>MKHLHRFFSSDASGGIILIIAAILAMIMANSGATSGWYHDFLETPVQLRVGSLEINKNMLLWINDALMAVFFLLVGLEVKRELMQGSLASLRQAAFPVIAAIGGMIVPTLLYLAFNYADPITREGWAIPAATDIAFALGVLALLGSRVPLALKIFLMALAIIDDLGAIIIIALFYTNDLSMASLGVAAVAIAVLAVLNLCGARRTGVYILVGVVLWTAVLKSGVHATLAGVIVGFFIPLKEKHGRSPAKRLEHVLHPWVAYLILPLFAFANAGVSLGGVTLDGLTSILPLGIIAGMLIGKPLGISLFCWLALRLKLAHLPEGTTYQQIMVVGILCGIGFTMSIFIASLAFGSVDPELINWAKLGILVGSISSAVIGYSWLRVRLRPSVGSENLYFQ[2x]

Na+/H+ exchangers facilitate the exchange of monovalent cations (Na+/Li+/K+) and protons (H+) across membranes to regulate intracellular pH, sodium levels and cell volume. Na+/H+ exchangers that perform this task are physiological homodimers, and whilst the ion transporting domain is highly conserved, their dimerization differs. The transporter is made up of two distinct domains, a dimerization domain and an ion-transporting (core) domain. Here, we report cryo-EM structures of E. coli NhaA and E. caballus NHE9 in complex with cardiolipin and phosphatidylinositol-3,5-bisphosphate PI(3,5)P2 lipids binding at their respective dimer interfaces.

Following sample preparation optimization, a data set of 14,329 movies was collected and a cryo-EM map at 3.3 Å resolution was calculated, according to the gold-standard Fourier shell correlation (FSC) 0.143 criterion. Similar to previous NhaA crystal structures, the cryo-EM structure of NhaA adopts the inward-facing conformation. As such, the mutation of charged residues on the cytoplasmic surface can alter the pH of NhaA activation and mutation of surface histidine residues to alanine abolished activity altogether. Similar to the monomeric crystal structure at pH 6.520, an intracellular cavity in the cryo-EM structure at pH 7.5 has opened to enable Na+ accessibility to the ion-binding site. The cryo-EM structure of NhaA is of the retained physiological homodimer. One CDL lipid (CDL 1) was located in the middle of the positively-charged part of the dimerization interface, flanked by two additional CDL lipids (CDL 2) bound at the ends of the dimer interface. Although this part of the dimerization interface is very positively-charged with four arginine side chains per protomer contributing — R203, R204, R245 and R250 — only the symmetry-related R204 residues directly interacts with the phosphate headgroups of the central CDL 1 lipid. Additional hydrogen bonds are contributed by T205 and W258 to oxygen atoms of the CDL 1 phosphoester bonds. The flanking CDL 2 lipids form hydrogen bonds to R204 and resides in a hydrophobic pocket lined by residues W258, Y261, and L262 from one protomer and L197, V207, and L210 from the other protomer. Here we could structurally confirm that CDL binds between the NhaA protomers and it is there stabilised by interactions with arginine residues. The structure of NhaA in complex with CDL supports the proposed regulatory switch induced by salt-stress in E. coli.>[3x]GHMPLLSASIVSAPVVTSETYVDIPGLYLDVAKAGIRDGKLQVILNVPTPYATGNNFPGIYFAIATNQGVVADGCFTYSSKVPESTGRMPFTLVATIDVGSGVT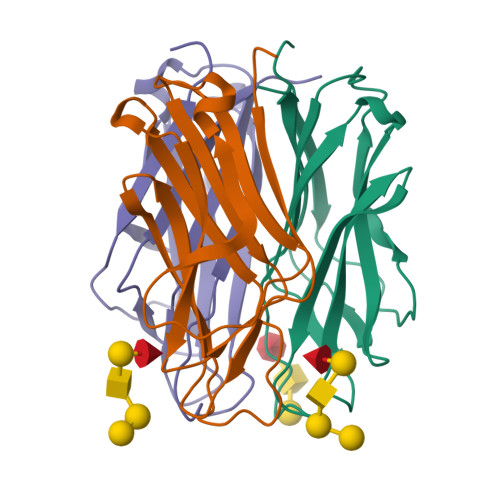FVKGQWKSVRGSAMHIDSYASLSAIWGTAA>MEFGSFLVSLGTSFVIFVILMLLFTWLSRKSGNAPIYYPNRILKGLEPWEGTSLTRNPFAWMREALTSSEQDVVNLSGVDTAVHFVFLSTVLGIFACSSLLLLPTLLPLAATDNNIKNTKNATDTTSKGTFSQLDNLSMANITKKSSRLWAFLGAVYWISLVTYFFLWKAYKHVSSLRAQALMSADVKPEQFAILVRDMPAPPDGQTQKEFIDSYFREIYPETFYRSLVATENSKVNKIWEKLEGYKKKLARAEAILAATNNRPTNKTGFCGLVGKQVDSIEYYTELINESVAKLETEQKAVLAEKQQTAAVVFFTTRVAAASAAQSLHCQMVDKWTVTEAPEPRQLLWQNLNIKLFSRIIRQYFINFFVAVTILFYMIPIAFVSAITTLKNLQRIIPFIKPVVEITAIRTVLESFLPQIALIVFLAMLPKLLLFLSKAEGIPSQSHAIRAASSKYFIFSVFNVFIGVTLAGTLFNTVKDIAKNPKLDMIINLLATSLPKSATFFLTYVALKFFIGYGLELSRIIPLIIFHLKKKYLCKTEAEVKEAWYPGDLSYATRVPGDMLILTITFCYSVIAPLILIFGITYFGLGWLVLRNQALKVYVPSYESYGRMWPHIHQRILAALFLFQVVMFGYLGAKTFFYTALVIPLIITSLIFGYVCRQKFYGG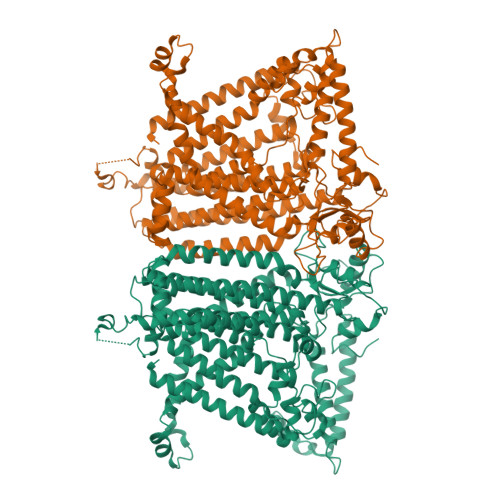FEHTALEVACRELKQSPDLEEIFRAYIPHSLSSHKPEEHEFKGAMSRYQDFNAIAGV[2x]>ACTWPAWEQFKKDYISQEGRVIDPSDARKITTSQGQSYGMFSALAANDRAAFDNILDWTQNNLAQGSLKERLPAWLWGKKENSKWEVLDSNSASDGDVWMAWSLLEAGRLWKEQRYTDIGSALLKRIAREEVVTVPGLGSMLLPGKVGFAEDNSWRFNPSYLPPTLAQYFTRFGAPWTTLRETNQRLLLETAPKG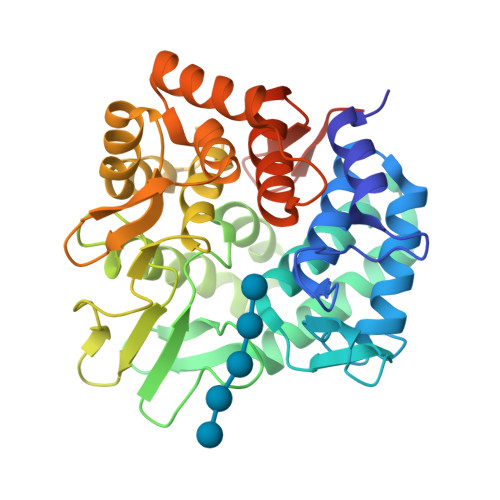FSPDWVRYEKDKGWQLKAEKTLISSYDAIRVYMWVGMMPDSDPQKARMLNRFKPMATFTEKNGYPPEKVDVATGKAQGKGPVGFSAAMLPFLQNRDAQAVQRQRVADNFPGSDAYYNYVLTLFGQGWDQHRFRFSTKGELLPDWGQECANSHLEHHHHHH[4x]> AASTT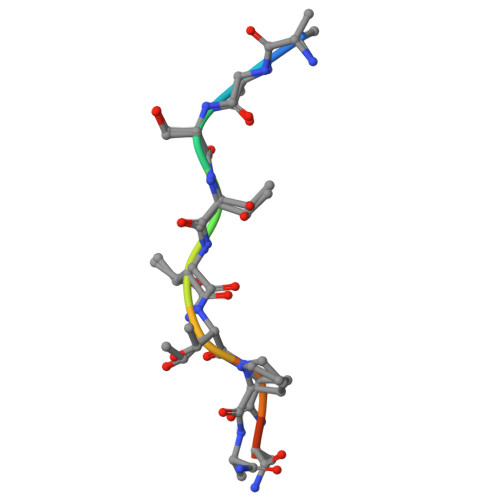TPAPA> GSHMASMKKKGSVVIVGRINLSGDTAYAQQTRGEEGCQETSQTGRDKNQVEGEVQIVSTATQTFLATSINGVLWTVYHGAGTRTIASPKGPVTQMYTNVDKDLVGWQAPQGSRSLTPCTCGSSDLYLVTRHADVIPVRRRGDSRGSLLSPRPISYLKGSSGGPLLCPAGHAVGIFRAAVSTRGVAKAVDFIPVESLETTMRSP

The HCV NS3/4A protease – a chymotrypsin-like serine protease – is a prime therapeutic target that cleaves four known sites along the virally encoded polyprotein. The NS3/4A protease also hydrolyzes two human proteins, TRIF and MAVS, which are part of the innate immune system, thereby confounding the innate immune response to viral infection. In this study, we report that four chemically representative protease inhibitors – telaprevir, danoprevir, vaniprevir and MK-5172 – exhibit distinct susceptibilities to the protease variants R155K, A156T and D168A. To elucidate the underlying mechanism by which chemically diverse inhibitors bind to the wild-type protease and drug-resistant variants, crystal structures were determined for 16 inhibitor-protease complexes. These complexes include wild-type protease and resistant variants R155K, D168A and A156T each bound to telaprevir, danoprevir, vaniprevir and MK-5172, with resolutions ranging from 1.10–2.50 Å; S139A protease variants were used except for telaprevir, which requires covalent bond formation with the serine 139 for efficient binding.

Boceprevir and telaprevir are two NS3/4A protease inhibitors recently approved by the Food and Drug Administration, marking an important milestone in anti-HCV research and drug development over the past two decades. Both boceprevir and telaprevir are linear ketoamide compounds that form a reversible, covalent bond with the catalytic serine of NS3/4A protease. Against wild-type protease, macrocyclic inhibitors danoprevir, vaniprevir and MK-5172 exhibited antiviral potencies in the sub nM range (IC50 = 0.24, 0.34 and 0.11 nM, respectively), while telaprevir potency was significantly lower (IC50 = 1030 nM), consistent with previous reports. The P5 amide nitrogen of telaprevir formed an additional hydrogen bond with the carbonyl oxygen of S159. In the telaprevir complex, the catalytic serine (S139) was covalently bound to the C-α carbon of the ketoamide warhead. The ketoamide oxygen sat in the oxyanion hole and interacted with the backbone amide nitrogens of protease residues 137–139, while the Nε nitrogen of H57 hydrogen bonded with the keto oxygen. The relatively weak binding affinity of telaprevir to wild-type protease results in a potentially narrow range by which resistant mutations can be tolerated.> LKDSLRPKLSEEQQHIIAILLDAHHKTYDPTYADFRDFRPPVRMDGSTGSVTLDLSPLSMLPHLADLVSYSIQKVIGFAKMIPGFRDLTSDDQIVLLKSSAIEVIMLRSNQSFTMDDMSWDCGSQDYKYDVTDVSKAGHTLELIEPLIKFQVGLKKLNLHEEEHVLLMAICIVSPDRPGVQDAKLVEAIQDRLSNTLQTYIRCRHPPPGSHQLYAKMIQKLADL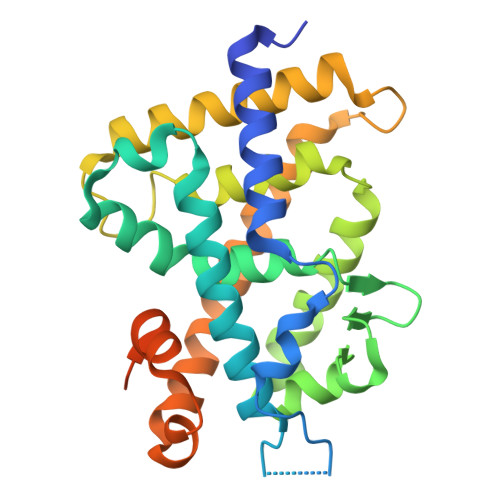RSLNEEHSKQYRSLSFQPENSMKLTPLVLEVFGNEISLVPRGSMAISDPNSSSVDKLAAALEHHHHHH4-[4-(1-methylpiperidin-4-yl)butyl]-~{N}-[6-(2-methylpropyl)quinolin-5-yl]benzenesulfonamide 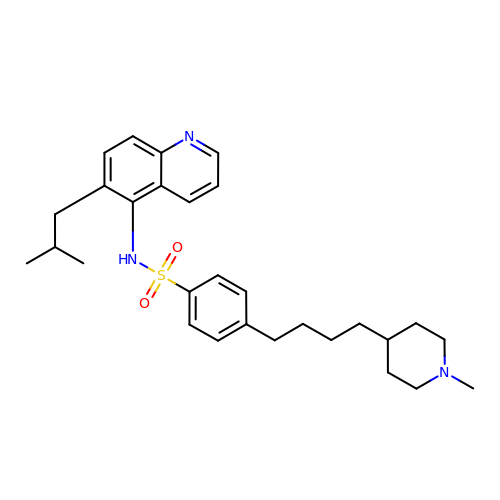| C29 H39 N3 O2 S | ZEJRJRISLHICJV-UHFFFAOYSA-N>[2x]GTMGKSKGTRFERDLLVELWKAGFAAI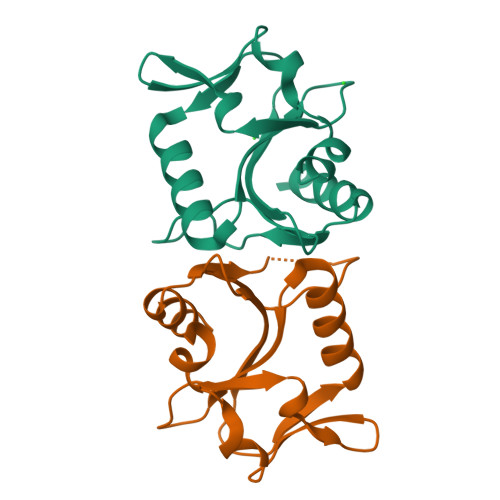RVAGSGVSPFPCPDIVAGNGRTYLAIEVKMRKELPLYLSADEVEQLVTFARGFGAEAYVALKLPRKKWRFFPVQMLERTEKNFKIDESVYPLGLEIAEVAGKFFQERFGEKV N-tert-butyl-2-[2-[6,6-dimethyl-8-(methylsulfonylamino)-11-oxidanylidene-naphtho[2,3-b][1]benzofuran-3-yl]ethynyl]-6-methyl-pyridine-4-carboxamide | C32 H31 N3 O5 S | 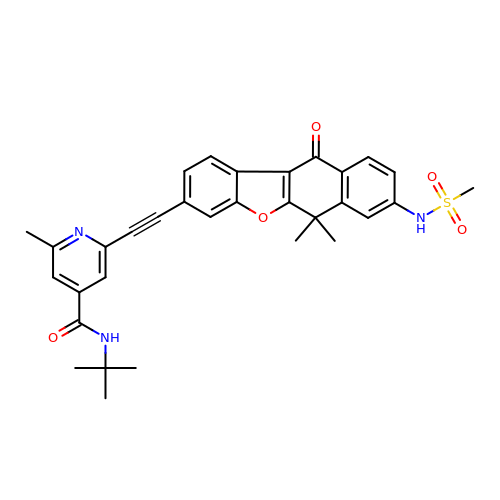DCGOHGQJHJXBGW-UHFFFAOYSA-N> GPHMSPDKKWLGTPIEEMRRMPRCGIRLPLLRPSANHTVTIRVDLLRAGEVPKPFPTHYKDLWDNKHVKMPCSEQNLYPVEDENGERTAGSRWELIQTALLNKFTRPQNLKDAILKYNVAYSKKWDFTALIDFWDKVLEEAEAQHLYQSILPDMVKIALCLPNICTQPIPLLAAAMNHSITMSQEQIASLLANAFFCTFPRRNAKMKSEYSSYPDINFNRLFEGRSSRKPEKLKTLFCYFRRVTAAAPTGLVTFTRQSLEDFPEWERCEKPLTRLHVTYEGTIEENGQGMLQVDFANRFVGGGVTSAGLVQEEIRFLINPELIISRLFTEVLDHNECLIITGTEQYSEYTGYAETYRWSRSHEDGSERDDWQRRCTEIVAIDALHFRRYLDQFVPEKMRRELNKAYCGFLRPGVSSENLSAVATGNWGCGAFGGDARLKALIQILAAAAAERDVVYFTFGDSELMRDIYSMHIFLTERKLTVGDVYKLLLRYYNEECRNCSTPGPDIKLYPFIYHAVESCAETADHSGQRTGT

PARG, a single gene alternatively spliced to generate five isoforms, is an endo- and exo-glycohydrolase that rapidly degrades PAR generated by PARP1 to coordinate DNA repair. PARG hydrolyzes α(1′′-2′) O-glycosidic linkages in PAR chains to release ADP-ribose and oligo(ADP-ribose) chains that may signal genotoxic stress. The hPARG active site has two deep pockets that specifically engage the adenine and diphosphate group of ADPR. Our high-resolution crystal structures of human PARG bound to these methylxanthine inhibitors revealed detailed interactions that support a mechanism of competitive inhibition.

The crystal structure of JA2-4 bound to hPARG refined at 1.7 Å resolution, identified a single JA2-4 molecule in the adenine-binding pocket. JA2-4 makes extensive site-specific interactions with hPARG, consistent with its potent inhibitory activity (IC50 of 0.9 μM). The methylxanthine head of JA2-4 makes π-stacking interactions with Phe902 side chain. The tail of JA2-4 extends from the 8´-position of the xanthine ring and is highly curved, which serves to make van der Waals contacts with Asn869. Structural superposition of hPARG bound to JA2-4 and ADP-HPD revealed that the methylxanthine core of JA2-4 occupies the same binding site as the adenine of ADP-HPD, consistent with a competitive block of substrate binding activity. Additionally, the 2´-carbonyl oxygen of JA2-4 hydrogen bonded with the main chain amide of Ile726. The most striking feature of the JA2-4 interaction with hPARG is a significant change in the Tyr clasp conformation. The JA2-4 binding site is obstructed by the side chain of Tyr795 in the unbound hPARG and in hPARG bound to ADP-HPD. To accommodate JA2-4, the Tyr795 side chain is flipped out from the adenine-binding pocket (with ~90° rotation), which positions the thioether of JA2-4 in contact with Cβ of Tyr795. Most notably, JA2-4 binding caused the Arg671 side chain to swing ~9 Å towards the tip of the Tyr clasp, where it makes an electrostatic interaction with Glu797 side chain and hydrogen bonds to the main chain carbonyl of Ala750 (not shown in this view).>SDEVRKNLMDMFRDRQAFSEHTWKMLLSVCRSWAAWCKLNNRKWFPAEPEDVRDYLLYLQARGLAVKTIQQHLGQLNMLHRRSGLPRPSDSNAVSLVMRRIRKENVDAGERAKQALAFERTDFDQVRSLMENSDRCQDIRNLAFLGIAYNTLLKIAEIARIRVKDISRTDGGRMLIHIGRTKTLVSTAGVEKALSLGVTKLVERWISVSGVADDPNNYLFCRVRKNGVAAPSATSQLSTRALEGIFEATHRLIYGAKDDSGQRYLAWSGHSARVGAARDMARAGVSIPEIMQA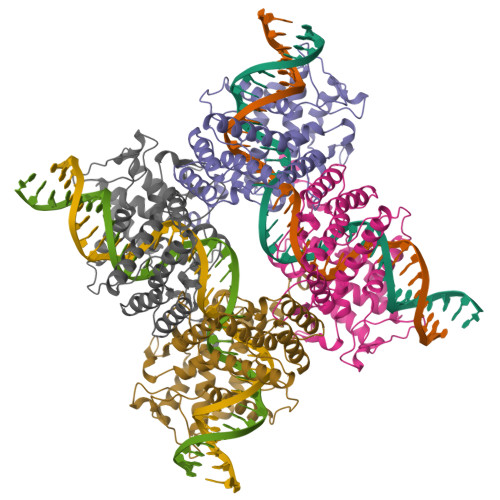GGWTNVNIVMNYIRNLDSETGAMVRLLED[2x]> MKTFIFLALLGAAVAFPVDDDDKIVGGYTCGANTVPYQVSLNSGYHFCGGSLINSQWVVSAAHCYKSGIQVRLGEDNINVVEGNEQFISASKSIVHPSYNSNTLNNDIMLIKLKSAASLNSRVASISLPTSCASAGTQCLISGWGNTKSSGTSYPDVLKCLKAPILSDSSCKSAYPGQITSNMFCAGYL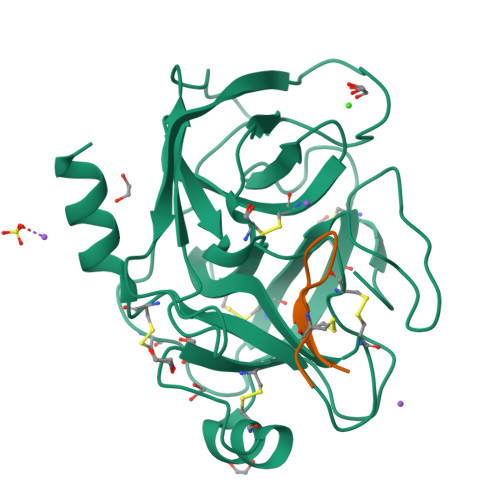EGGKDSCQGDSGGPVVCSGKLQGIVSWGSGCAQKNKPGVYTKVCNYVSWIKQTIASN;> GRCTKSIPPICFP> PVDMSNLFYKTLLDDFSRSLEMQPLVFDDHGTCNMIIDNTFALTLSCDYARERLLLIGLLEPHKDIPQQCLLAGALNPLLNAGPGLGLDEKSG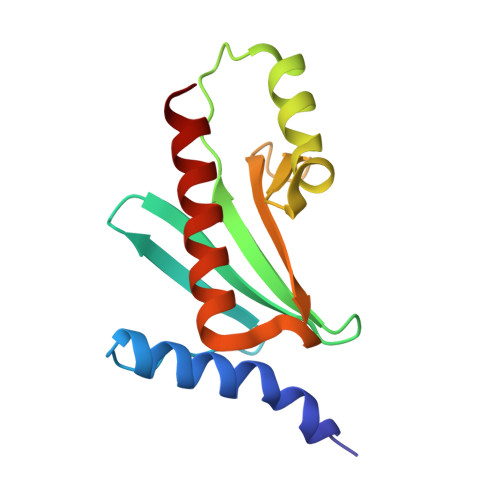LYHAYQSIPREKLSVPTLKREMAGLLEWMRGWREA> MNLTDSLQNVLSGVGTLNRYRLDIPSCPSSLDVEDFSGTEGISKIYRYDIIFTSTDRYPDAAWFLRKSATLIMGTGLLESLTEQKKVHGVITDFRRISGSEDQAQYRITLKPFISLLDKQFRTHRFFVNKSVPEVVEQILTEHGLKGWEYEFSLKRTYPKREQINQYQESDLRFIQRLLAEVGIFYFFTLHPDAQTEVIHFGDVQAALIFDKTLPVNSPSGMSDSGTDSVWALNVEHRVVESRVITNDYNHREAQNILMSVPADMTRGEGYDTSYGEVYHYRPRHTERGDKIDPAPETANFWARLDHERFLAEQTRITGKSTDASLLPAQVLTITDSTPPVLPAPLQEPVLLTQLLFTGSRKSALQVMLSAVPYSEIVCWRPPLLTRPKITGTMTARVTSAKEGDIYAWQDASGMYRVKFDADRDDKNPGQESMPVRLAKPYSGDAYGFHFPL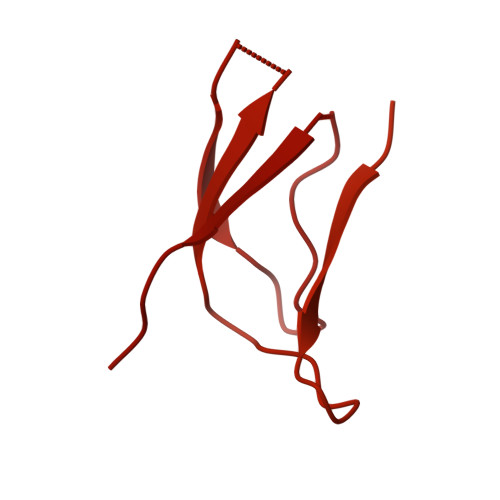IQGTEVAIAFEEGDPDRPYIAHALHDSRHVDHVTDKNGTRNVIRTPANNKLRMEDKRGEEHIKLSTEYGGKTQLNLGHNVDASRELRGEGAELRTDDWISIRGGKGIFISADMQPQAQGKMLDMDEAIRQLEQALSLARSMAKAATAANATQGDISCQQRLNASLTDLTAPGMLLHAPDGIGMVSARALRIASGSESVGIMSGDNTDITAGQSFTVVAEGAVSLLSRNQGMQLLAAKGRVNIQAQSDDLSMSSQQNLDIQSSEGKVTVSANQELILACGGAYIKLSGGNIELGCPGQILLKSTNMQKMGPTSLDIASVEMPRGFGGGFILTDEAGVPQPSTPYRLTTAEGDILQGITDENGKTAPVNTSIPSVVKVEFGKVKIHGETE> MSQSKSGGAVGPFNSVAEAAGCVATTDWMLLVLLFFAVLGGYHVHFMLTAGDWDFWVDWKDRRMWPTVLPILGVTFCAASQAFWWVNFRLPF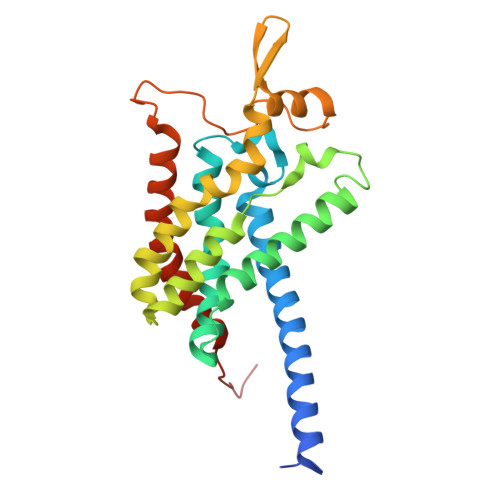GAVFAVLGLMIGEWINRYVNFWGWTYFPISLVFPSAMIVPAIWLDVILLLSGSYVITAVVGSLGWGLLFYPNNWPAIAAFHQATEQHGQLMTLADLIGLHFVRTSMPEYIRMVERGTLRTFGKDVVPVAAFFSGFVSMMVYFLWWFMGRWYSTTKRIEQI>MSQGFDDEFGGADQYDTPLSHLRLTARLNTSALDSRRGVVRLHPEVLAALGIREWDAVALTGTRTTAAVAGVAGPGVPAGTALLDDVTLSNAGVRENAAVLVSPVTVYGARSVTVSGSRLATQSISPATLRMALLGKVMTVGDTVSLLPRDLGPGTSTSAATSALASSVGITWTSELLTVTAVDPPGTVSVQPNSVVSWGTGTPEDPAPPPTGRHTVSPQRSEQPVSFDDVKVTHPQAVKLDEWLRLSLDEPELLKTLGATPHLGVLVSGPAGVGKATMVRAVCASRRVVELDGPEVGALQVDERLRSVTSAVAAVTESGGVLFIADVDALLPAGNEMRPPEPVATLILAELRKAVATPGVAFIATSAVPENVDARLRAPEVCDRELGLSLPDATARRSLLEMLLRGVPSEDLDLGDIADHTPGFVVADLAAVVREGALRAAARASSSDDDPVLRHADLEGALTVIRPLSRSASEEVSVGSVTLDDVGDMVETKRALTEAVLWPLQHPDTFSRLGIDPPRGVLLYGPPGCGKTFVVRALASSGRLSVHAVKGSELMDKWVGSSEKAVRELFARARDSAPSLVFLDEIDALAPRRGQNFDSGVTDKVVASLLTELDGIEPLRDVVVLGATNRPDLIDPALLRPGRLERLVFVEPPDAAARRDILRTAGKSIPLADDVDLDSLADDLDGYSAADCVALLRESAMTAMRRSIDAADVTAADVAKARETVRPS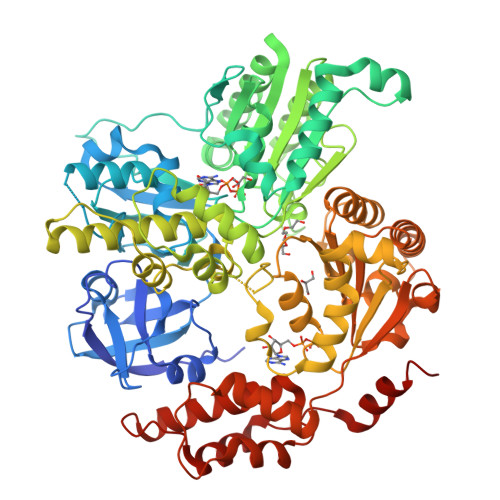LDPAQVESLREFAEKR[2x]>MSLKYFKRLSDRERAIFEAG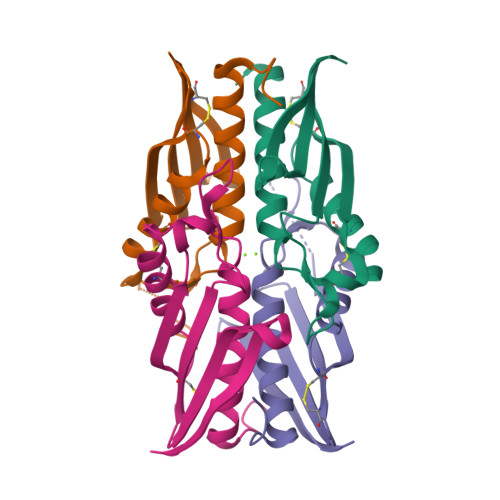ITLGAIYHQFCGTPVSPGTAEEVAKCIERAALLQPCVIDARVEVDVSSEDTDNYGGYTEVSGRNLRVTIVTRCGEWEAVGKLEFIEELNYPLMWVEEIRRVEQEGHHHHHH[4x]4-methoxycyclohexa-2,5-diene-1-thione | C7 H10 O S | 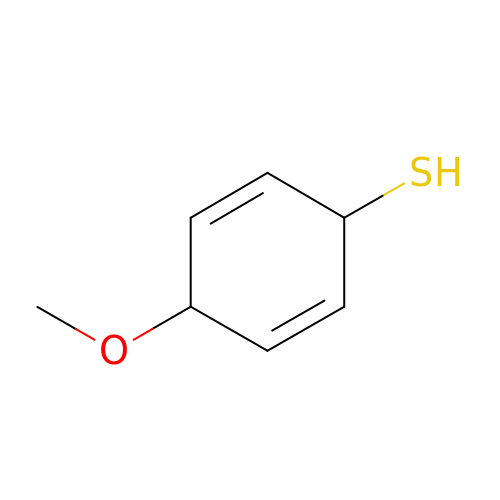ODGVEVKXIQCVID-KNVOCYPGSA-N> MAHHHHHHMTSVGLIWAQSTSGVIGRDGGIPWRLPEDLAHFKRLTMGHTVVMGRRTWDSLPAAHRPLPGRRNVVVTRQTGLVAHGAQVVGSLE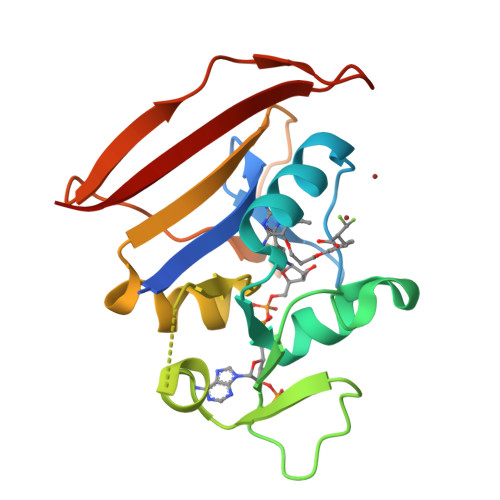QALSPAEPDAETWVIGGAQIYALALPLANRCEVTEVDVDLPPEDEDALAPVLDQTWAGTSGEWLVSRSGLRYRMHSYRRL> GPYDIGDELGRGTQGITYHAVERSSGDNYAAKIMYGRPELRPFMLNELEMMNTFNHKNLIRPYDAYDTDRSVTLIMELAAGGELVRDNLLRRDYYTERDIAHYIRQTLWGLEHMHEMGVGHMGLTIKDLLISVVGGDIIKVSDFGLSRKINRHNLSTLDYGMPEFVSPEVVNKEGVNFSHDMWTVGLITYVLLGGHNPFLGIDDRETLTKIREGRWDFKDEIWTHISDDGRDFISRLLLYSPEERMDVKTALKHPWFFMLDRPVYDHDYQIGTDRLRNYYDHFRDWYANASCKNYFR

Obscurins are large filamentous proteins with crucial roles in the assembly, stability and regulation of muscle. Characteristic of these proteins is a tandem of two C-terminal kinase domains, PK1 and PK2, that are separated by a long intrinsically disordered sequence. Our study of PK1 from Drosophila obscurin shows that this is a pseudokinase with features typical of the CAM-kinase family, but which carries a minimalistic regulatory tail that no longer binds calmodulin or has mechanosensory properties typical of other sarcomeric kinases. PK1 binds ATP with high affinity, but in the absence of magnesium and lacks detectable phosphotransfer activity.

Of the variants tested, only the protein construct encompassing the kinase domain followed by 40 C-terminal residues (dmUNC89/Obsc residues 3186–3480) yielded a soluble and stable protein product viable for structural analysis. The atomic structure of dmObsc-PK1 was then elucidated to 1.75 Å resolution using X-ray crystallography. The structure revealed the kinase domain followed by a short CRD tail, limited to the first regulatory helix, αR1 (nomenclature as in 18), with the remaining 8 terminal residues being poorly ordered in electron density maps. Helix αR1 is amphipathic and its packing against the kinase is mediated by a cluster of aromatic residues that includes the conserved tryptophan W3469 at the helix C-terminus. The overall structure of dmObsc-PK1 resembles that of other CAM-kinases, e.g. DAPK, which also displays a CRD tail that is disordered beyond helix αR1. However, this disinhibited state of dmObsc-PK1 -where ATP and substrate binding sites are exposed- contrasts markedly with structures of nearest homologues, the sarcomeric titin-like kinases. In dmObsc-PK1, both the catalytic (C)-spine (residues I3199, A3213, L3267, L3312, L3313, I3314, I3371, L3375) and the regulatory (R-)spine (residues M3234, P3245, H3304, F3327) are pre-formed in the absence of ATP binding. Finally, in dmObsc-PK1, the activation loop is in an open state so that access to the active site is unrestricted. In summary, these features indicate that dmObsc-PK1 adopts an overall conformation similar to that of canonical kinases in the active state. More globally, nucleotide binding does not induce either global or local conformational changes in dmObsc-PK1, with apo and ADP-complexed crystal structures being equivalent (RMSDCα = 0.18Å).7-(3,4-dimethoxyphenyl)-6-methylquinazoline-2,4-diamine 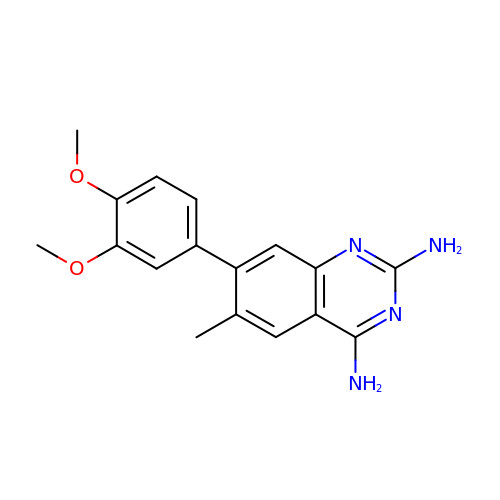| C17 H18 N4 O2 | UGJMRAQTQALEME-UHFFFAOYSA-N>DDLSGFKKIKLGELELFILTDGYIHEENLISFAPRGNVAELKTILKDNFRADHYIDMAINILLVKTKEKLILMDTGMGIFADERTGFLLKSLQKAGFSAHDITDIFLSHAHPDHIGGVVDKQNKLVFPNASIFISKIEHDFWINASIKDFNNSALKAHPE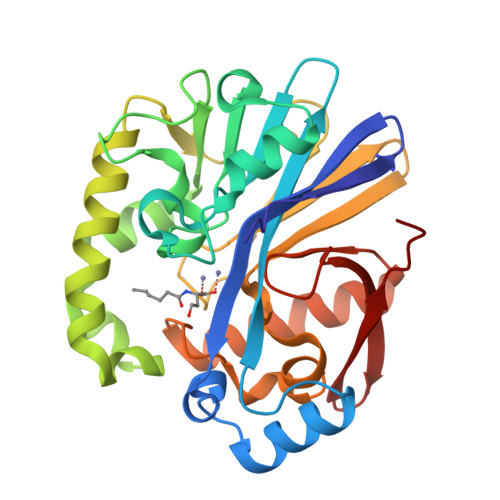RLNQIIPALQNILKAIQPKLKFYDLNKTLYSHFNFQLAPGHTPGLTVTTISSGNEKLMYVADLIHSDVILFPHPDWGFSGDTDLDIATASRKKFLKQLADTKARAFTSHLPWPGLGFTKVKAPGFEWIPESFMN[2x]>MPAMKIECRITGTLNGVEFELVGGGEGTPEQGRMTNKMKSTKGALTFSPYLLSHVMGYGFYHFGTYPSGYENPFLHAINNGGYTNTRIEKYEDGGVLHVSFSYRYEAGRVIGDFKVVGTGFPEDSVIFTDKIIRSNATVEHLHPMG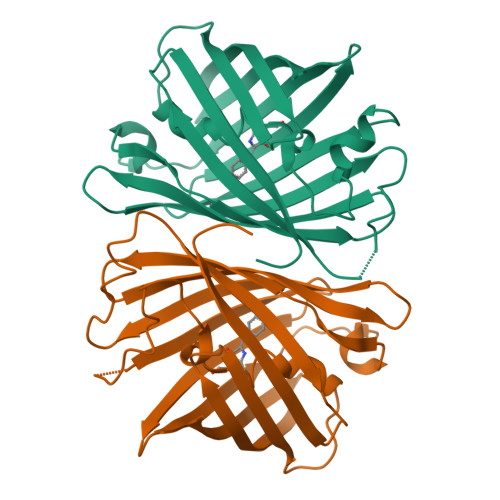DNVLVGSFARTFSLRDGGYYSFVVDSHMHFKSAIHPSILQNGGPMFAFRRVEELHSNTELGIVEYQHAFKTPIAFA[6x]4-METHYLCATECHOL | C7 H8 O2 | 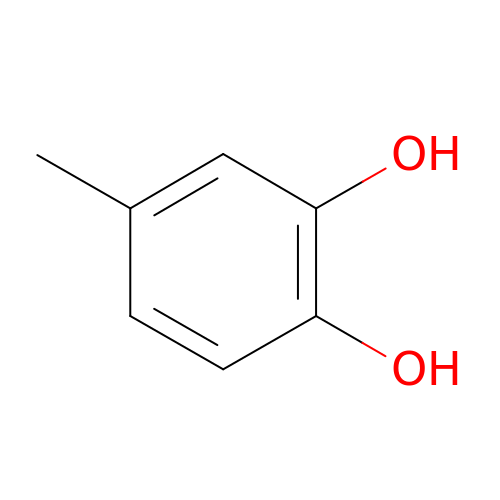ZBCATMYQYDCTIZ-UHFFFAOYSA-N>GCATGCATGC[4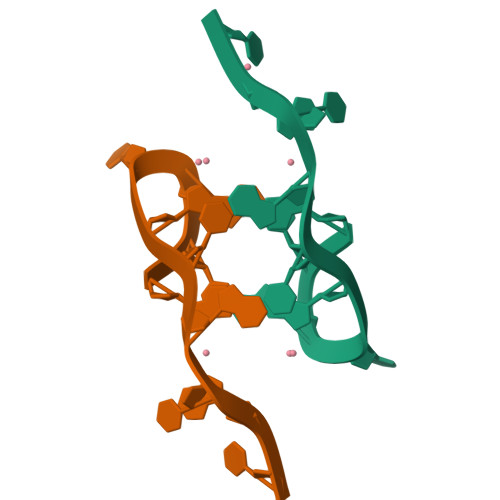x]> MEIVEYPDPILRAKNKRIDIFDENLKNLVDAMFDVMYKTDGIGL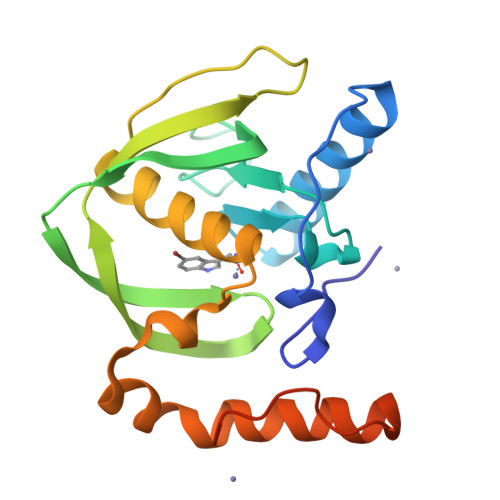SAPQVGLNVQLMVFNPAGEPGEGKEIVLVNPKIKKYSDKLVPFDEGCLSFPGIYAEVVRPQSVKIDARDITGERFSISLSRLPARIFQHEYDHLEGVLFFDRMTDQVLDSIREELEALEKKYEEKTGLPSPERVEARQKRKAGVGFGKR Sorcin is one of the most highly expressed calcium-binding proteins in many tissues, and part of the 5% most expressed proteins of the human proteome (PaxDb). Importantly, Sorcin is overexpressed in many human tumors and MDR cancers. Upon calcium binding Sorcin undergoes a large conformational change that exposes three pockets, hydrophobic surfaces involving the EF loop and EF5 hand (Pocket 1), EF2-EF3 (Pocket 2) and region EF1-EF3 (Pocket 3). This allows Sorcin to bind and regulate target proteins in a calcium-dependent fashion.

Here we demonstrate that Sorcin binds doxorubicin directly and with high affinity and that it changes its cellular localization upon doxorubicin treatment and limits the toxic effects of doxorubicin in the cell; the low resolution structure of Sorcin in complex with doxorubicin allowed the identification of at least one chemotherapeutic drug binding site. The asymmetric unit contains two dimers (A–B and C–D). The structure contains 10 Mg2+ ions (3 bound to monomer A, 2 to monomer B, 3 to monomer C, 2 to monomer D). Doxorubicin is bound to the B monomer. The superimposition between the Cα trace of doxo-SCBD with the Cα trace of apo-Sorcin yields an rmsd of 1.11 Å, indicating that the structures are similar and therefore neither Mg2+ ions binding nor doxorubicin binding are able to promote the conformational changes induced by calcium ions in Sorcin. Inspection of the Fo-Fc electronic density map allowed the identification of two peaks: one close to the EF5 hand, which does not bind calcium in Sorcin and is responsible for dimer formation, and the other close to the D-helix connecting the EF2 and EF3 sites at the interface between the two dimers. We succeeded in modeling the doxorubicin molecule in the first site (close to the EF5) whereas it was not possible to model the doxorubicin molecule in the second site (close to the D helix) indicating both the low occupancy of the site and the flexibility of the doxorubicin molecule. The binding of doxorubicin to SCBD in pocket 1 involves a stacking interaction of the drug with the aryl ring of Tyr188 of one monomer and interaction with Asp177, Gly182, Phe173 and Phe134 of the two-fold symmetry related monomer at the dimeric interface. In the second putative site (pocket 2) doxorubicin likely interacts with Trp105 and Phe134. In the structure, magnesium is bound to EF3 and to part of EF1 and EF2 sites, showing that in Sorcin the first three EF-hands can bind not only calcium, but also magnesium, with rather high affinity, and that EF3 is the site endowed with the highest affinity for divalent cations, responsible for Sorcin cation-dependent activation.

>MDPLYGYFAAVAGQDGQIDADELQRCLTQSGIAGGYKPFNLETCRLMVSMLDRDMSGTMGFNEFKELWAVLNGWRQHFISFDTDRSGTVDPQELQKALTTMGFRLSPQAVNSIAKRYSTNGKITFDDYIACCVKLRALTDSFRRRDTAQQGVVNFPYDDFIQCVMSV[4x]> MSVLVSGATGFIAQHIVNVLLEQNYKVIGTVRSQEKADKLIKQFNNNPNLSFEIVPDIANLDAFDEVFKKHGKEIKYVIHTASPVHFGTTDYEKDLLIPAVNGTKGILESIKKYAPDTVERVVITSSFAAIMDLNKQSDSSVIFTEKSWNPVTWENAQNAITAYCGSKTFAEKAAWDFLKENKDSVKFKLTTINPVFVFGPQLFDEDVKDKLNTSCEIINELLHAPPDTKVDKSSTCAGNFIDVRDVAKAHVLAFQKDELIGKRLLLSNGPFSKQDIVNILNKDFPQLKGKIPPADPDTDAQKNNTTGCKIDNEKTKKLLGFEFKSFEETVYDTVHQILKK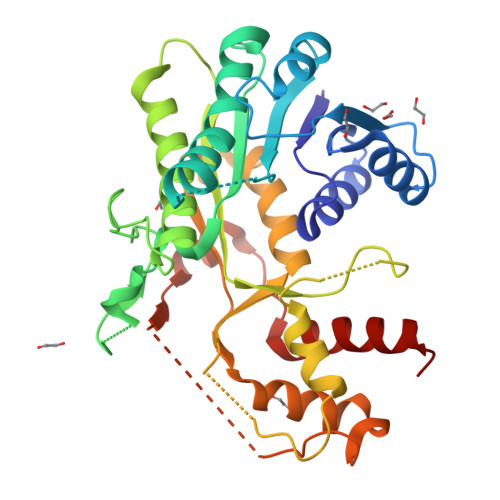EGKL[(2~{R},5~{R})-5-[(5-fluoranylpyridin-2-yl)oxymethyl]-2-methyl-piperidin-1-yl]-(5-methyl-2-pyrimidin-2-yl-phenyl)methanone 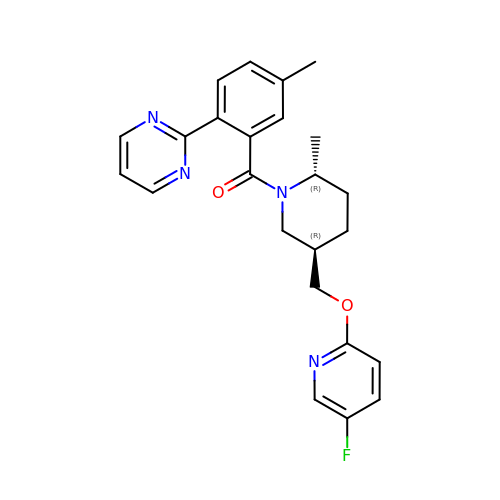| C24 H25 F N4 O2 | NPFDWHQSDBWQLH-QZTJIDSGSA-N>[4x]GHMENSLNALSQEALYKNWLTSRCIGKSTDSE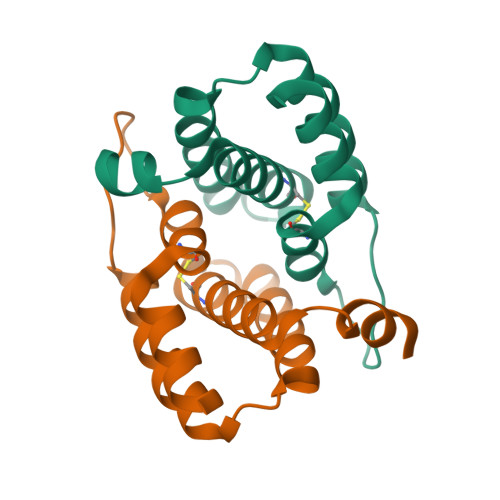RTKQDAFRSASAYLELSKLPMDAFEQGEKLAEQYANKNSQGSVQGTYHTLDCLSLQNASEAETIFERYSK> GIDPFTGEAIAKFNFNGDTQ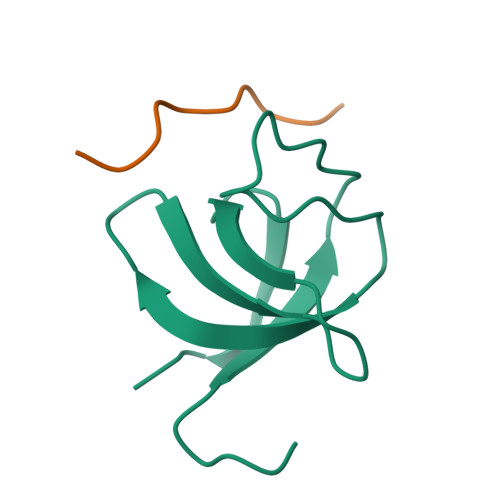VEMSFRKGERITLLRQVDENWYEGRIPGTSRQGIFPITYVDVIKRPL;> VPPPVPPPPS> SNAMRLVADSACDIKELRGMVFKAVPLTISTDNEEFCDDGQLDIHRMLDILEKHKGRSYTACPGIDAWLEAFGDDDEIFVVTITAGMSGTYNSAMAARAVYLEEHPQAKVRVIDSKSTGPQMRIILEQLQQMIEEGK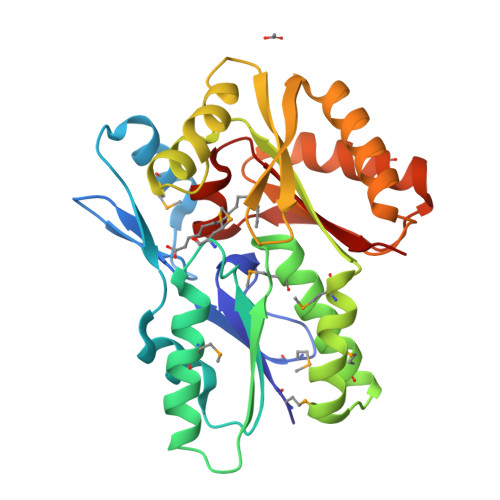KFEEIDGAIDAYMQKTRLFCSLKSLHNLAQNGRVSKVVASAAEVLGISVIGTASSHGTLEAIGKCRGDKKLLVKLQALLDDAGYEGGKLRICHVENEALADKIADMIKQAYGTTDVCVYKAGGLCSYYAERGGIILSCETK> MVAKGRIIRVTGPLVVADGMKGAKMYEVVRVGELGLIGEIIRLEGDKAVIQVYEETAGVRPGEPVVGTGASLSVELGPGLLTSIYDGIQRPLEVIREKTGDFIARGVTAPALPRDKKWHFIPKAKVGDKVVGGDIIGEVPETSIIVHKIMVPPGIEGEIVEIAEEGDYTIEEVIAKVKTPSGEIKELKMYQRWPVRVKRPYKEKLPPEVPLITGQRVIDTFFPQAKGGTAAIPAPFGSGKTVTQHQLAKWSDAQVVIYIGCGERGNEMTDVLEEFPKLKDPKTGKPLMERTVLIANTSNMPVAAREASIYTGITIAEYFRDMGYDVALMADSTSRWAEALREISGRLEEMPGEEGYPAYLASKLAEFYERAGRVVTLGSDYRVGSVSVIGAVSPPGGDFSEPVVQNTLRVVKVFWALDADLARRRHFPAINWLTSYSLYVDAVKDWWHKNIDPEWKAMRDKAMALLQKESELQEIVR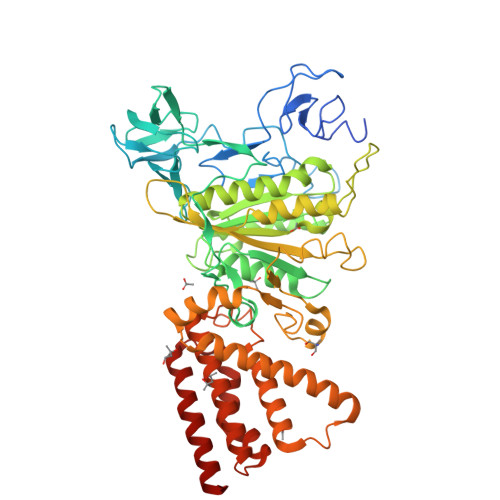IVGPDALPERERAILLVARMLREDYLQQDAFDEVDTYCPPEKQVTMMRVLLNFYDKTMEAINRGVPLEEIAKLPVREEIGRMKFERDVSKIRSLIDKTNEQFEELFKKYGA> HGEKSQAAFMRMRTIHWYDLSWSKEKVKINETVEIKGKFHVFEGWPETVDEPDVAFLNVGMPGPVFIRKESYIGGQLVPRSVRLEIGKTYDFRVVLKARRPGDWHVHTMMNVQGGGPIIGPGKWITVEGSMSEFRNPVTTLTGQTVDLENYNEGNTYFWHAFWFAIGVAWIGYWSRRPIFIPRLLMVDAGRADELVSATDRKVAMGFLAATILIVVMAMSSANSKYPITIPLQAGTMRGMKPLELPAPTVSVKVEDATYRVPGRAMRMKLTITNHGNSPIRLGEFYTASVRFLDSDVYKDTTGYPEDLLAEDGLSVSDNSPLAPGETRTVDVTASDAAWEVYRLSDIIYDPDSRFAG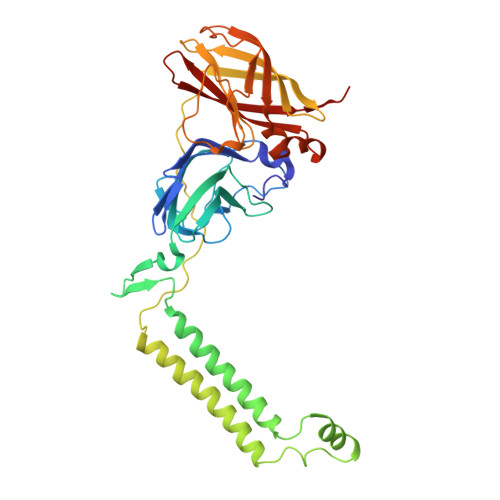LLFFFDATGNRQVVQIDAPLIPSFM> MSAPTDDTPTDAIAAPRHSAPPRPRLPWFLRTFAVPIILAWVAVVAILNTVVPTLDEVGEMRAVSMAPNDAPSTLAIKRVGQVFEEYDTSSSVMIVLEGEEPLGIEAHAFYDKMVADLRADTEHVQHVQDFWGDTLTASGAQSVDGKAAYVQVYIAGDQGESLANESVEAVRKIATERETPSGVKAYVTGAAATSADQRAEGDASMKLIEGVTFAVITVMLLAVYRSVITTLIVLAMVVLGLSGARGIVAFLGFYNVFGLTTFATNMVVTLAIAAATDYAIFLIGRYQEARRAGEDRESAYYTMFHGTAHVVLASGLTIAGATLCLHFTRLPYFQTMGVPLAIGMLIVVAAALTAGPAVISVVSRFGKTLEPKRFSRSPGWHRVGTATVRWPGAILVCAVVAALIGLLALPGYYTTYDDRRYLPDDVPANVGYDAAFRHFSQAKMNPDLMMVETDRDLRNPADFLV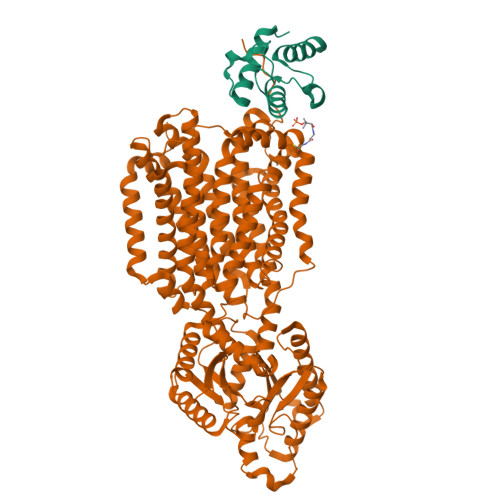IDKIAKALKNVHGIAQVQTITRPDGDPIEHSTIPYTIGQSGTTQIMNNDYMQTNLDNLLKQADDLQTSIDSMTEMMNIQTELAAVSQSMADKMAQTSDDTADVRDHLADFDDFFRPIRNYLYWEPHCYDIPMCWSMRSIFESIDGINTMSDDFQELVPEMRRMADLMPRMVAVMPAQIQSMKNQKQTLLNQYQVQKAQQDQNMAMQENATAMSQAFDAAKNDDSFYLPPEAFETDDFQRGMKLFMSPDGHAVRFTIIHQGDPLTEEGTARMDELKVAAADAIKGTPFEGARIYLGGSAATYNDMQIGADYDLIIVAASALILIFIIMMVLTRAVVAAAVIVGTVVLSLASAFGLSVLLWQHIVGIPLHWMVLPMSVIVLLAVGADYNLLLVSRMKEEIHAGIRTGIIRAMVGTGAVVTAAGLVFAFTMASMAVSSLITIGQVGTTIGLGLLFDTLVVRSLMTPSIATLLGRWFWWPQRVRERPVPSKWPTPIQRTPEEALS;> MAATQEEIIAGLAEIIEEVTGIEPSEVTPEKSFVDDLDIDSLSMVEIAVQTEDKYGVKIPDEDLAGLRTVGDVVAYIQKLEEENPEAAAALREKFAADQ>ADKELKFLVVDDFSTMRRIVRNLLKELGFNNVEEAEDGVDALNKLQAGGYGFVISDWNMPNMDGLEL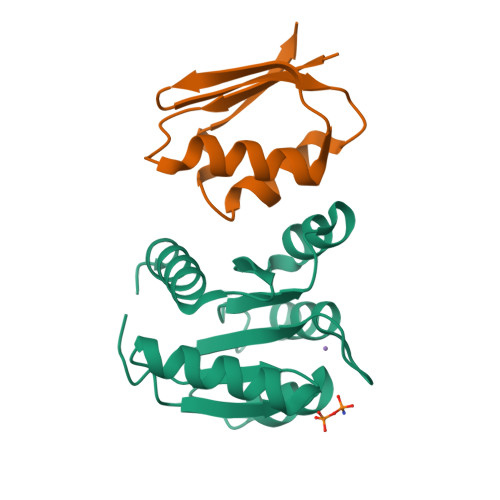LKTIRADGAMSALPVLMVTAEAKKENIIAAAQAGASGYVVKPFTAATLEEKLNKIFEKLGM[2x];>RQLALEAKGETPSAVTRLSVVAKSEPQDEQSRSQSARRIILSRLKAGEVDLLEEELGHLTTLTDVVKGADSLSAILPGDIAEDDITAVLCFVIEADQITFETVEVSPKISTPPVLKLAAEQAPTGRVEREKTTR[2x]4-(imidazo[1,2-a]pyridin-2-yl)benzene-1,2-diol 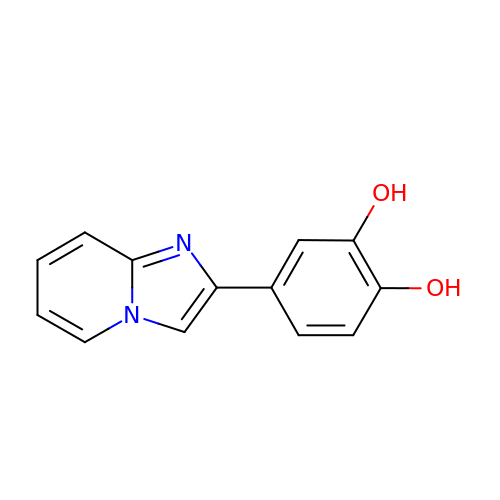| C13 H10 N2 O2 | JFYGSKNPLRBMMG-UHFFFAOYSA-N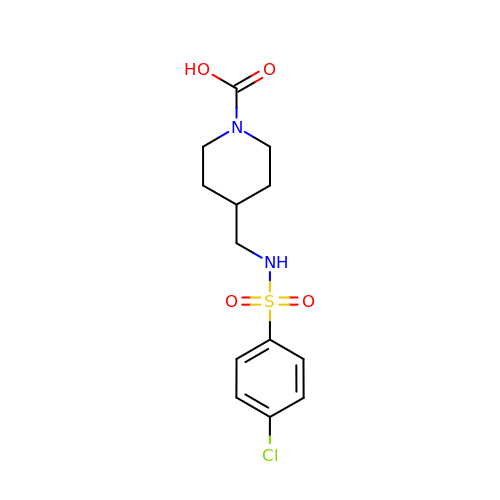4-({[(4-chlorophenyl)sulfonyl]amino}methyl)piperidine-1-carboxylic acid | C13 H17 Cl N2 O4 S | CFNWARLITZSZQR-UHFFFAOYSA-N(2R)-2-(pyridin-3-yl)-1-azabicyclo[2.2.2]octane 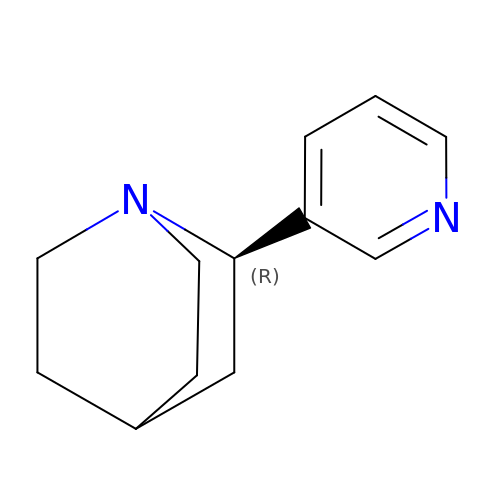| C12 H16 N2 | YJYPZLAZNIGNRP-GFCCVEGCSA-N>[4x]GPGAYISLNYHSPTIGMHQNLTVILPEDQSFFNSDTTVKPLKTLMLLHGLSSDETTYMRYTSIERYANEHKLAVIMPNVDHSAYANMAYGHSYYDYILEVYDY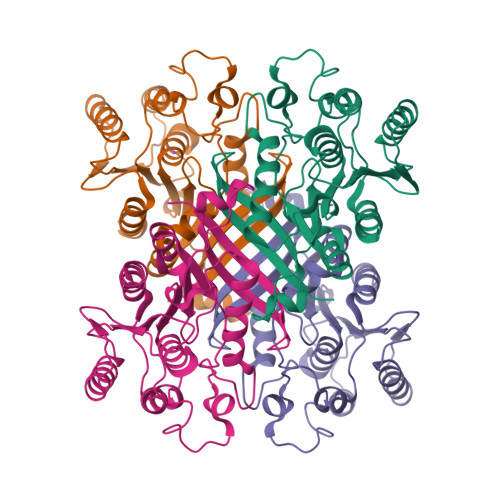VHQIFPLSKKRDDNFIAGHSMGGYGTIKFALTQGDKFAKAVPLSAVFEAQNLMDLEWNDFSKEAIIGNLSSVKGTEHDPYYLLDKAVAEDKQIPKLLIMCGKQDFLYQDNLDFIDYLSRINVPYQFEDGPGDHDYAYWDQAIKRAITWMVND Basement membranes are extracellular structures of epithelia and endothelia that have collagen IV scaffolds of triple α-chain helical protomers that associate end-to-end, forming networks. At the C-termini, interactions occur between the trimeric NC1 domains of two protomers, forming a hexamer of these domains reinforced by sulfilimine cross-links. Recent studies in one of our laboratories revealed that the NC1 domains function as recognition modules, directing the selection and assembly of α-chains into protomers and networks.

In an attempt to visualize the Goodpasture antigens, we tried to crystallize the α345NC1 heterohexamer by using an equimolecular mixture of pure recombinant α3NC1, α4NC1 and α5NC1 domains. Using this approach, while attempting to produce crystals of the α345NC1 heterohexamer that predominates in the BM of the kidney, we solved the three-dimensional structure of the recently reported homohexamer of α5NC1 domains. Size-exclusion chromatography experiments confirmed a strong tendency of α5NC1 to hexamerize: ∼80% of this domain was self-organized as hexamers in solution, while isolated α3NC1 or α4NC1 eluted as monomers. Conversely, our experimental results have shown that equimolecular mixtures of α3NC1, α4NC1 and α5NC1 only produce α5NC1homo crystals. Chloride ions were also present in our α1NC1homo, α3NC1homo and α5NC1homo structures at two different positions in the protomer–protomer interface. Our crystal structures of the α3NC1 and α5NC1 homohexamers provide the first view of the arrangement of the EA and EB regions, which are known critical components of two epitopes that reside in the dissociated α3 and α5 subunits of native α345NC1 hexamers. In the homohexamers these regions are exposed on the surface and are presumably unreactive to antibody binding, as they are in the native α345NC1 hexamers. In Goodpasture’s disease autoantibodies directed to the α3NC1 and α5NC1 domains are generated. In Alport’s syndrome, mutations in these chains, including α5NC1, lead to a defective network assembly, causing the multi-laminar splitting of the glomerular BM.

> SVAHGFLITRHSQTTDAPQCPQGTLQVYEGFSLLYVQGNKRAHGQDLGTAGSCLRRFSTMPFMFCNINNVCNFASRNDYSYWLSTPEPMPMSMQPLKGQSIQPFISRCAVCEAPAVVIAVHSQTIQIPHCPQGWDSLWIGYSFMMHTSAGAEGSGQALASPGSCLEEFRSAPFIECHGRGTCNYYANSYSFWLATVDVSDMFSKPQSETLKAGDLRTRISRCQVCMKRT> MNAIGNFLVGTPVFTIFICLALGYLLGKLKIGSFTLGATVGVLIVALLIGQLGVFPRDTLLGDIFFDFFMFAIGYRVGPSFISSMKKFGAKIVYATLIFLVSAFIVAYACFKMFHIGPGIAAGIIAGGLTQSAVIGSSLETISKLPISDHLKTLYSNQIPIVYTLTYVFGTIGVLIFLRDIMPKLMHIDLKKQAVKTAKELDMIPVPVIVASTHFYTINDGSSLIGQTLGTVNTKFAKGLVAAGLNDSADMASVINAGDVLAISGGIDEIGRAVQEFNLLEVTGKTKAYVSKQVVLKKNFSADVLKNAQDKGVLVATLAGDVMDPAQFSTLHHHHHHKPAESVTLVGQKDAVSEVQSQLGRLRAAENIINYSWFALGIALSAALGIVGTKVSGVPIALGGGTASLIVGLVQSIYRDKHAHMDTIPDSLLEFFQSIGLNLFIATVGLS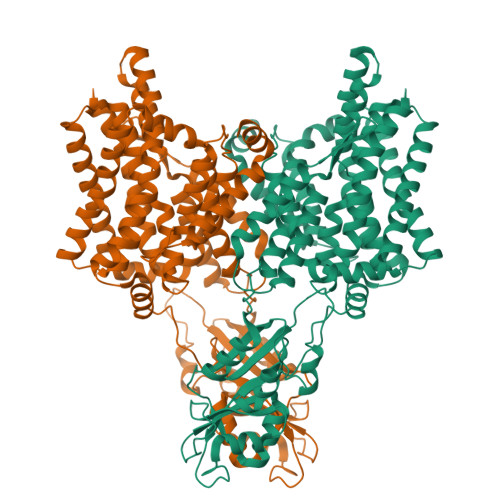AAKTFISAIQSMGISVLLIGAVISILPHIITFVICYYLMKMEPISIIGAQTGADTLSAALNDVSERVGSDASPFFAAAVAPAYAIGNIFLTLMGPIFIVLLS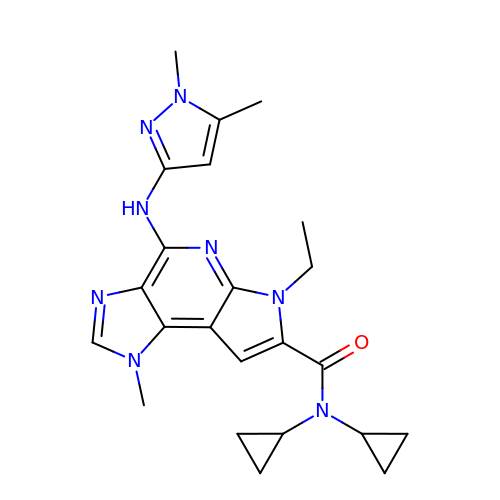N,N-dicyclopropyl-4-[(1,5-dimethyl-1H-pyrazol-3-yl)amino]-6-ethyl-1-methyl-1,6-dihydroimidazo[4,5-d]pyrrolo[2,3-b]pyridine-7-carboxamide | C23 H28 N8 O | JCINBYQJBYJGDM-UHFFFAOYSA-N> MGSSHHHHHHSSGENLYFQGSHMTATATSAKAAAPACPRFDDPVHAAADPRVDVERITPDPVWRTTCGTLYRSDSRGPAVVFEQGFLPKDVIDGQYDIESYVLGNQPSPYVSTTYDHDLYKTWYKSGYNYYIDAPGGVDVNKTIGDRHKWADQVEVAFPGGIRTEFVIGVCPVDKKTRTEKMSECVGNPHYEPWH

S. scabies produces a 200-residue, 22-kDa protein that is a single-domain enzyme called Scabin. Scabin has been cloned, expressed, and purified, and shown to harbor dual enzymatic activities (GH and ADP-ribosyltransferase). Scabin targets DNA as a substrate for ADP-ribose modification; it also shows enzyme specificity towards genomic DNA from Solanum tuberosum tubers. Scabin shares nearly 40% sequence identity with the Pierisin family of mARTs.

Scabin active-site residues proposed to interact with the ds-DNA substrate include Val109, Asn110, Gln111, Thr127, Trp128, Tyr129, Trp155, and Gln158 (DNA I strand); and Gln100, Asp102, Glu104, Ser105, Leu108, Tyr129, Lys130, Lys180, Lys181, and Arg183 (DNA II strand). The α2 residues, Leu108, and Val109 showed importance for both catalytic activities, with the former being more important for GH activity while the latter was more important for ADP-ribosyltransferase activity. The rest of the Scabin variants showed either a WT-like crystal structure or similar CD spectra to the WT in solution. All the structures were of high quality, ranging from 1.5 to 1.75 Å.>SMSTKGTILVTGGAGYIGSHTAVELLAHGYDVVIADNLVNSKREAIARIEKITGKTPAFHETDVSDERALARIFDAHPITAAIHFAALKAVGESVAKPIEYYRNNLDSLLSLLRVMRERAVKRIVFSSSATVYGVPERSPIDETFPLSATNPYGQTKLMAEQILRDVEAADPSWRVATLRYFNPVGAHESGLIGEDPAGIPNNLMPYVAQVAVGKLEKLRVFGSDYPTPDGTGVRDYIHVVDLARGHIAALDALERRDASLTVNLGTGRG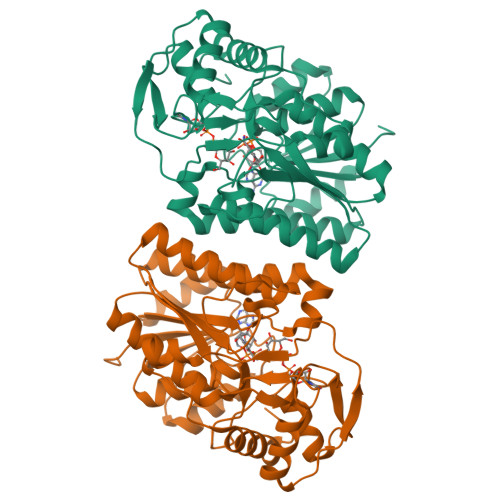YSVLEVVRAFEKASGRAVPYELVARRPGDVAECYANPAAAAETIGWKAERDLERMCADHWRWQENNPRGFV[2x]> MSSVDVLLTVGKLDASLALLTTQDHHVIEFPTV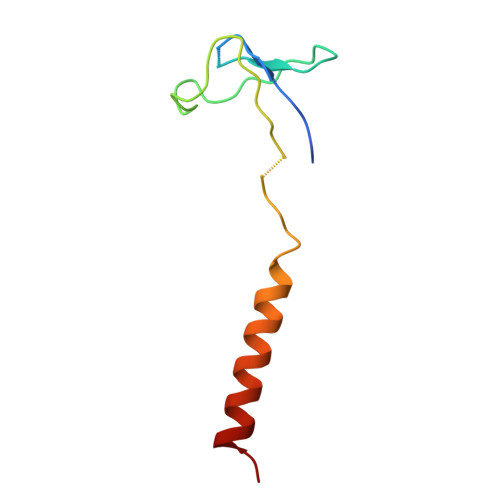LLPENVKAGSIIKMQVSQNLEEEKKQRNHFKSIQAKILEKYGTH>[2x]MAHHHHHHIPAPRLMWLYRNGDKHDDGTPFFVRPYIKSMESLYQQITKEITPIAGPVRRIFDQNFRVITDLDDIVDGAKYLCTSGEPPAAYDRLEKFLSEWVIQ

TgDCX is a doublecortin-domain protein associated with the conoid fibers, a set of strongly curved non-tubular tubulin-polymers in Toxoplasma. TgDCX contains two tubulin-binding domains: a partial P25α and the DCX/doublecortin domain. Previously we reported that TgDCX is specifically localized to the conoid in Toxoplasma, and that without TgDCX, the conoid structure becomes short and disordered, invasion of host cells is severely compromised, and the parasite forms many fewer and much smaller plaques relative to wild-type Toxoplasma. TgDCX alone has the unique ability of generating short, curved, and stable tubulin-containing polymers with a consistent curvature.

The sequence conservation among the TgDCX orthologues is mostly restricted to the predicted P25α and doublecortin domains. Both the full-length TgDCX and the TgDCX71–243 fragment are insoluble in non-denaturing buffer systems, but we were able to purify and crystallize a soluble fragment (AA148–243) that contains the DCX domain and determine its structure by X-ray crystallography. The fold of TgDCX148–243 is very similar to that of the N-terminal DCX domain of human doublecortin, which itself is quite similar (root mean square distance (rmsd) of ~ 2 Å) to the doublecortin C-terminal DCX domain [HsDCX-N and HsDCX-C,]. Residues responsible for the four tubulin contact regions between HsDCX-N and tubulin identified by structural docking are in most cases similar. Given the high level of homology among the TgDCX orthologues in the region of their DCX domains, we used the structure of TgDCX148–243 as a model for threading the corresponding regions in the TgDCX orthologues in Chromera velia (CvDCX1, CvDCX2, CvDCX3), Vitrella brassicaformis (VbDCX1, VbDCX2, VbDCX3), Plasmodium falciparum (PfDCX), and Trichoplax adhaerens (TaDCX). At the location reported in [9] corresponding to tubulin contact region #3 in HsDCX-N (K53), which abuts a strongly electronegative patch on β-tubulin, orthologues that bind efficiently to microtubules have a positive charge (R152 in TgDCX, lysine in CvDCX1 and PfDCX), whereas most of the orthologues that do not bind have isoleucine. The comparison of orthologues also revealed a reversal of polarity at one position: D201 in TgDCX and D at the corresponding location in CvDCX1 and PfDCX, is replaced by K or R at the corresponding residue in CvDCX2, CvDCX3, VbDCX2, VbDCX3, and TaDCX. Both sidechains however are orientated away from the microtubule, indicating that they are not directly involved in tubulin binding. Indeed, mutations at these two residues in TgDCX (R152I_D201R) and in a non-binding orthologue CvDCX2 (I85R_R134D) do not appreciably decrease TgDCX binding to microtubules nor increase CvDCX2 binding in Xenopus S3 Cells. When expressed in Toxoplasma (whether in the wild-type or in the TgDCX knockout background), mCherryFP-TgDCX148–243 was not enriched in the conoid.Tripartite ATP-independent periplasmic (TRAP) transporters are a large family of SBP-dependent secondary-active transporters that are found exclusively in prokaryotes to catalyze the uptake of a variety of substrates, primarily organic anions, across the cytoplasmic membrane. A defining feature of TRAP transporters is the obligate utilization of an SBP, which is either found in the periplasm or attached to the outer leaflet of the cytoplasmic membrane, where it binds and delivers the substrate to the membrane component. Here, we have characterized VcGluP, a TAXI TRAP SBP from V. cholerae, the first experimentally validated glutamate transporter identified in this pathogen. We have shown that VcGluP preferentially binds glutamate and can also bind glutamine with a micromolar affinity.

To investigate the selectivity determinants of VcGluP, we solved the structure of VcGluP in the presence of excess (0.5 mM) L-glutamate to 1.7 Å, using molecular replacement. The refined model obtained in the presence of 0.5 mM L-glutamate contains residues 29–328, which equates to all of the 299 residues of mature VcGluP. VcGluP is composed of 2 α/β domains connected by a hinge composed of antiparallel β-sheets (residues 116–131 and 255–267). Comparison with other SBP structures reveals that VcGluP belongs to Cluster F. In addition, each domain contains a disulfide bond; Cys53–Cys67 in domain 1 which connects a1 with B2, and Cys191–Cys216 in domain 2 that connects a8 and a9, although density for this disulfide is missing likely through radiation damage. We also identified three Na+ ions bound to the surface of the protein (purple spheres and Fig. S2), although due to their distance from the binding site, we predict that these are functionally irrelevant interactions and merely a consequence of the 2.4 M sodium malonate used during crystallization. During refinement, we identified non-protein density in the cleft between the two domains, which we assigned to L-glutamate, which was present at 0.5 mM during crystallization. As expected, in the presence of ligand, VcGluP adopts a closed conformation wherein the two domains completely envelope the ligand binding site. Analysis of the ligand binding site reveals that L-glutamate is coordinated by VcGluP via a hydrogen bonding network composed of direct mainchain and sidechain interactions, and indirectly through coordinated water molecules. The α-carboxyl group of the bound L-glutamate makes sidechain and mainchain interactions with S75, mainchain interactions with G156 and hydrogen bonds to a water molecule, which is itself coordinated by the D157 sidechain. However, we found that binding affinity was only severely diminished when Y45 and Q93 were mutated to alanine, reducing the affinity by 213- and 990-fold, respectively, suggesting that these residues are the key binding determinants for VcGluP.

> RAQDFITIGTGSVTGVYYPTGGAICKLVNKDRKDHNIRCSVESTGGSIYNVNTIRSGELDFGIVQSDWQYHGYNGTSEFAEQGPYKKLRAVFSMHTEPFNIIARADSGIENVKDLAGKRVNIGNPGSGDRATMQVVMDAFGWNNDSFKLAAELKGSERSQALCDNKIDAFIYMVGHPNGAIKEATTSCAAKLVPATGPEIEKIVANNPYYAYSVVPAGMYSGTDQEVKSFGVAATLVTTEEVSEAVVYNLTKAVFENFDTFTRLHPAFANLKKEDMVTAGNSIPLHPGAVKYYKEAGLIK>[3x]PPGPP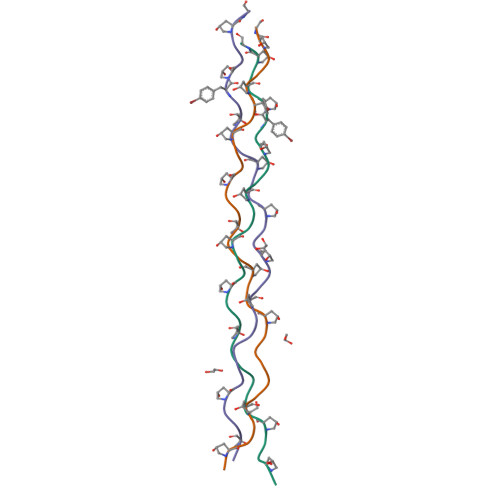GPRGPPGPPGVPGPPGPPGYPGPPGX> KGPAEDTYSTSWTNVNYASDSLESHNLDIYLPKEQKTAYKAIIIIYGSAWFANNAKAMASASIGAPLLKAGFAVISINHRSSMEAIWPAQIQDVKAAIRYVRSNAAKYNIDPSFIGITGFSSGGHLSAFAGVTNGVKTLTSGDLTVDIEGSLGNYLSTGSHVDAVVDWFGPVDMAHMSNCVAPNDASTPEAVLIGKKDPREEPDWVKLISPINFVDKDDPDILIIHGDADNVVPHCQSVNLKNVYDNAGAKATFISVPGGGHGPGCFDTQYFKDMTDFFTEQSTKLEHHHHHH

BD-FAE, a previously unknown protein encoded in a metagenomic PUL from beaver droppings belongs to the functionally diverse α/β-hydrolase superfamily. We demonstrated that BD-FAE removes feruloyl and acetyl groups from simple model substrates, acetyl groups from birchwood glucuronoxylan, and feruloyl groups from highly substituted AcFaXOS from corn fiber. The His-tag was not visible and the N-terminal tail showed weaker electron density than other residues of the protein, most likely due to its flexible protruding nature. Overall, the BD-FAE crystal structure adopted a typical α/β-hydrolase fold, which was consistent with the above mentioned BLASTp results. The active center contained the conserved catalytic triad of Ser128, Asp237 and His269 and the oxyanion hole was composed of NH-groups of Gly53 and Ser128.

The final model of the truncated form was refined to 1.85 Å resolution and contained residues from Met8 to Lys292. Surprisingly, also in the crystal of the truncated form, higher-order oligomers were observed indicating that N-terminal deletion was not sufficient for disrupting this assembly. Surprisingly, the crystal structure of an N-terminal truncated form of BD-FAE (∆Met1-Pro7) adopted a similar spiral shaped polymer. The interaction surface area of sequential molecules in the truncated form, however, was determined to be 764 Å2, which is 28% smaller compared to BD-FAE (1055 Å2). In the crystal structure of the truncated form, the serine protease inhibitor AEBSF (4-(2-aminoethyl)benzenesulfonyl fluoride) of the lysis buffer covalently bound to the active site’s Ser128. The phenolic ring in bound AEBS moiety resembled the binding of ferulic acid and tetrahedral sulfonyl of Ser-AEBS mimicked the enzyme–substrate–intermediate during carboxylic acid binding at Ser128. Based on that observed complex structure, Araf substituted with a 5-O linked feruloyl residue (Fa-Araf), a common substituent of xylans, was successfully docked into the active site of BD-FAE. The amino acid residues that bound Fa-Araf in BD-FAE were similar to those binding the AEBS moiety, and were in a long α-helical loop after the β5 strand. A stabilizing disulfide bond between Cys186 and Cys242 prevented extensive movement of that loop. The hydroxyl group of ferulic acid bound in BD-FAE to Glu197 in a bidentate way.NAPHTHALENE-2,6-DISULFONIC 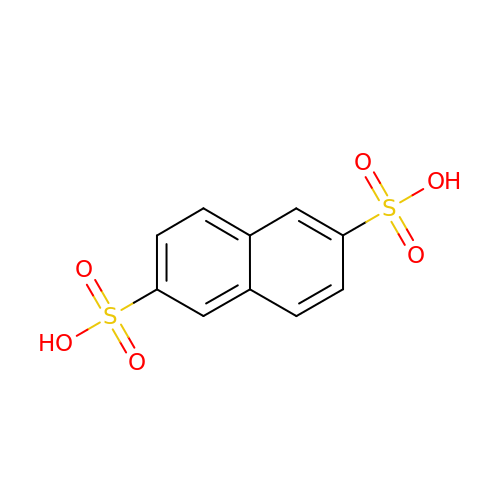ACID | C10 H8 O6 S2 | FITZJYAVATZPMJ-UHFFFAOYSA-N> EHTWPDKGSLYIATTHTQARYALPGVIKGFIERYPRVSLHMHQGSPTQIAEAVSKGNADFAIATEALHLYDDLVMLPCYHWNRSIVVTPDHPLAATSSVTIEALAQYPLVTYTFGFTGRSELDTAFNRAGLTPRIVFTATDADVIKTYVRLGLGVGVIASMAVDPLADPDLVRIDAHDIFSHSTTKIGFRRSTFLRSYMYDFIQRFAPHLTRDVVDTAVALRSNEEIEAMFQDIKL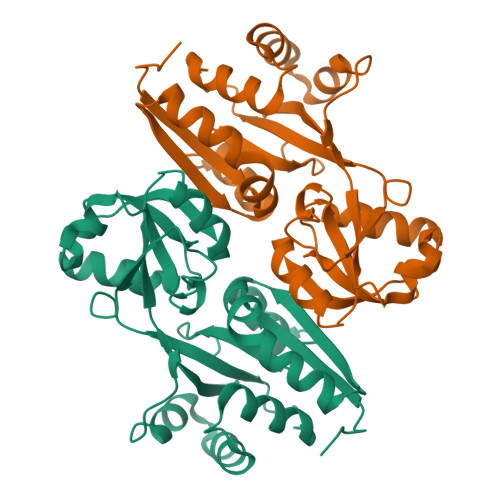PEK> MERTNTTTFKFFSLGGSNEVGRSCHILQYKGKTVMLDAGIHPAYQGLASLPFYDEFDLSKVDILLISHFHLDHAASLPYVMQRTNFQGRVFMTHPTKAIYRWLLRDFVRVTSIGSSSSSMGTKDEGLFSDEDLVDSFDKIETVDYHSTVDVNGIKFTAFHAGHVLGAAMFQIEIAGLRVLFTGDYSREVDRHLNSAEVPPLSSNVLIVESTFGTATHEPRLNRERKLTQLIHSTVMRGGRVLLPVFALGRAQEIMLILDEYWSQHAD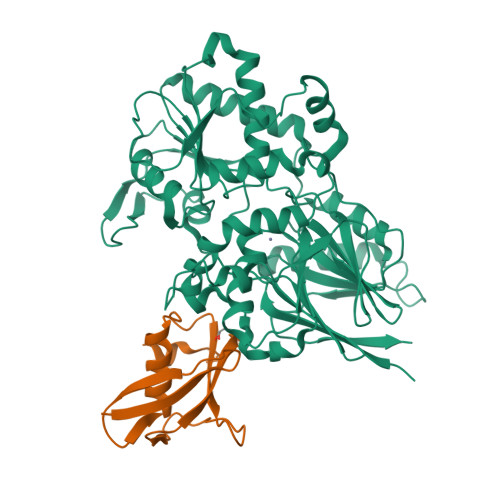ELGGGQVPIFYASNLAKKCMSVFQTYVNMMNDDIRKKFRDSQTNPFIFKNISYLRNLEDFQDFGPSVMLASPGMLQSGLSRDLLERWCPEDKNLVLITGYSIEGTMAKFIMLEPDTIPSINNPEITIPRRCQVEEISFAAHVDFQENLEFIEKISAPNIILVHGEANPMGRLKSALLSNFASLKGTDNEVHVFNPRNCVEVDLEFQG;> MSSTIFYRFKSQRNTSRILFDGTGLTVFDLKREIIQENKLGDGTDFQLKIYNPDTEEEYDDDAFVIPRSTSVIVKRSPAIKSFSVHSRLKGNVGAAAKGNATRYVTGRPRVLQKRQHTATTTANVSGTTEEERIASMFATQENQWEQTQEEMSAATPVFF>[20x]MALSKVKLNDTLNKDQLLSSSKYTIQRSTGDSIDTPNYDVQKHINKLCGMLLITEDANHKFTGLIGMLYAMSRLGREDTIKILRDAGYHVKANGVDV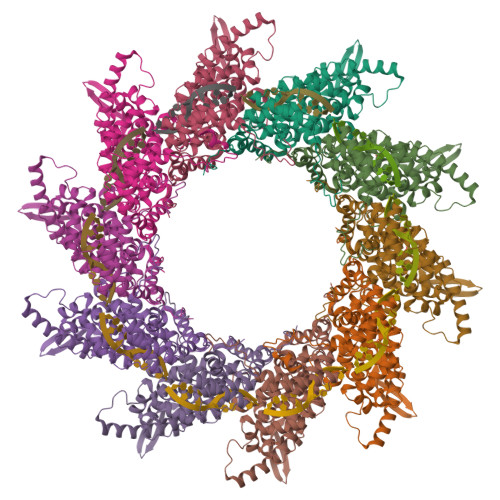TTHRQDINGKEMKFEVLTLASLTTEIQINIEIESRKSYKKMLKEMGEVAPEYRHDSPDCGMIILCIAALVITKLAAGDRSGLTAVIRRANNVLKNEMKRYKGLLPKDIANSFYEVFEKHPHFIDVFVHFGIAQSSTRGGSRVEGIFAGLFMNAYGAGQVMLRWGVLAKSVKNIMLGHASVQAEMEQVVEVYEYAQKLGGEAGFYHILNNPKASLLSLTQFPHFSSVVLGNAAGLGIMGEYRGTPRNQDLYDAAKAYAEQLKENGVINYSVLDLTAEELEAIKHQLNPKDNDVEL> MSFESKKPMRTWSHLAEMRKKPSEYDIVSRKLHYSTNNPDSPWELSPDSPMNLWYKQYRNASPLKHDNWDAFTDPDQLVYRTYNLM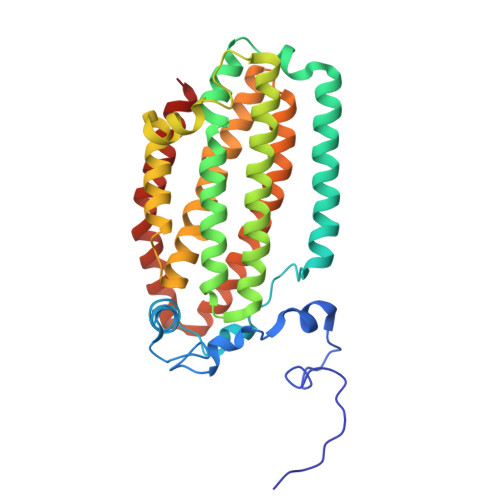QDGQESYVQSLFDQFNEREHDQMVREGWEHTMARCYSPLRYLFHCLQMSSAYVQQMAPASTISNCCILQTADSLRWLTHTAYRTHELSLTYPDAGLGEHERELWEKEPGWQGLRELMEKQLTAFDWGEAFVSLNLVVKPMIVESIFKPLQQQAWENNDTLLPLLIDSQLKDAERHSRWSKALVKHALENPDNHAVIEGWIEKWRPLADRAAEAYLSMLSSDI> GDNYADLSDTELTTLLRRYNIPHGPVVGSTRRLYEKKIFEYETQRRRLSPPSSSAASSYSFSDLNSTRGDADMYDLPKKEDALLYQSKGYNDDYYEESYFTTRTYGEPESAGPSRAVRQSVTSFPDADAFHHQVHDDDLLSSSEEEC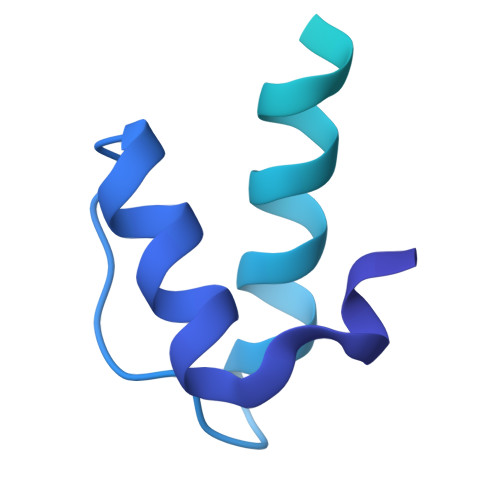KDRERPMYGRDSAYQSITHYRPVSASRSSLDLSYYPTSSS4-cycloheptyl-6-(3-piperidin-1-ylpropyl)pyrimidine-2-carbonitrile | C20 H30 N4 | 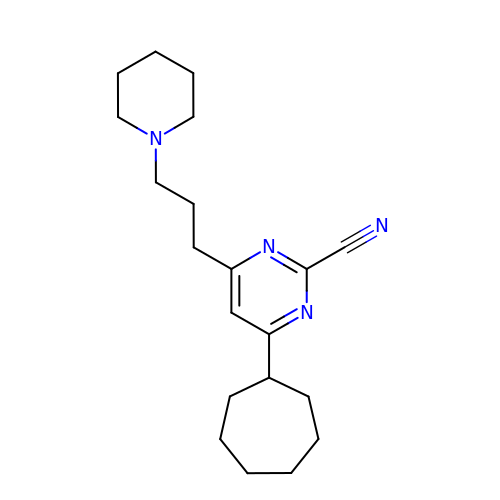UTNIKRVBYGTXDR-UHFFFAOYSA-N> MALISQSIKNLKGGISQQPDILRYPDQGSRQVNGWSSETEGLQKRPPLVFLNTLGDNGALGQAPYIHLINRDEHEQYYAVFTGSGIRVFDLSGNEKQVRYPNGSNYIKTANPRNDLRMVTVADYTFIVNRNVVAQKNTKSVNLPNYNPNQDGLINVRGGQYGRELIVHINGKDVAKYKIPDGSQPEHVNNTDAQWLAEELAKQMRTNLSDWTVNVGQGFIHVTAPSGQ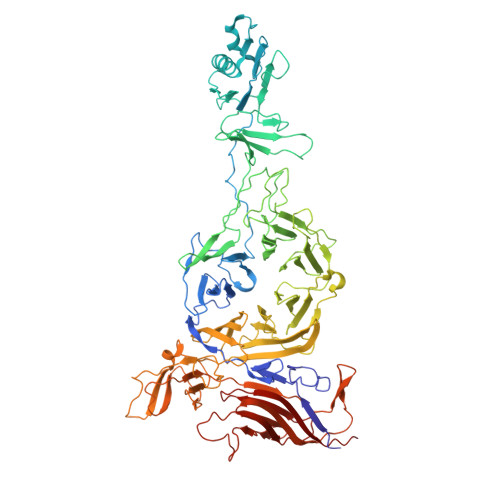QIDSFTTKDGYADQLINPVTHYAQSFSKLPPNAPNGYMVKIVGDASKSADQYYVRYDAERKVWTETLGWNTEDQVLWETMPHALVRAADGNFDFKWLEWSPKSCGDVDTNPWPSFVGSSINDVFFFRNRLGFLSGENIILSRTAKYFNFYPASIANLSDDDPIDVAVSTNRIAILKYAVPFSEELLIWSDEAQFVLTASGTLTSKSVELNLTTQFDVQDRARPFGIGRNVYFASPRSSFTSIHRYYAVQDVSSVKNAEDITSHVPNYIPNGVFSICGSGTENFCSVLSHGDPSKIFMYKFLYLNEELRQQSWSHWDFGENVQVLACQSISSDMYVILRNEFNTFLARISFTKNAIDLQGEPYRAFMDMKIRYTIPSGTYNDDTFTTSIHIPTIYGANFGRGKITVLEPDGKITVFEQPTAGWNSDPWLRLSGNLEGRMVYIGFNINFVYEFSKFLIKQTADDGSTSTEDIGRLQLRRAWVNYENSGTFDIYVENQSSNWKYTMAGARLGSNTLRAGRLNLGTGQYRFPVVGNAKFNTVYILSDETTPLNIIGCGWEGNYLRRSSGI>GSHMSNTQTVLPFTGLNTPSG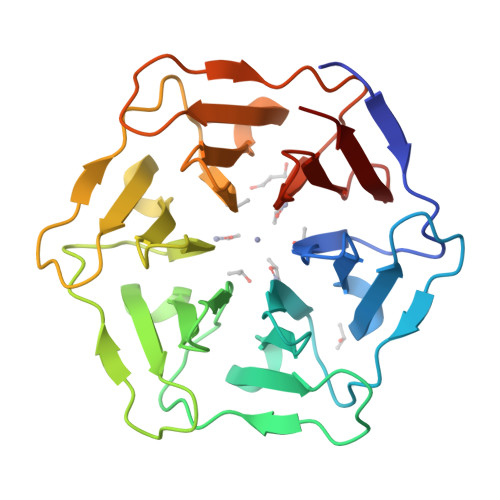VAVDSAGTVYVTDHGNNRVVKLAAGSTNQVTLPFTGLNTPHGVAVDSAGTVYVTDHGNNRVVKLAAGSNTQTVLPFTGLNTPSGVAVDSAGTVYVTDHGNNRVVKLAAGSTNQVTLPFTGLNTPHGVAVDSAGTVYVTDHGNNRVVKLAAGSNTQTVLPFTGLNTPSGVAVDSAGTVYVTDHGNNRVVKLAAGSTNQVTLPFTGLNTPHGVAVDSAGTVYVTDHGNNRVVKLAAG[2x]> GSHMSSLPVPYKLPVSLSVGSCVIIKGTPIHSFINDPQLQVDFYTDMDEDSDI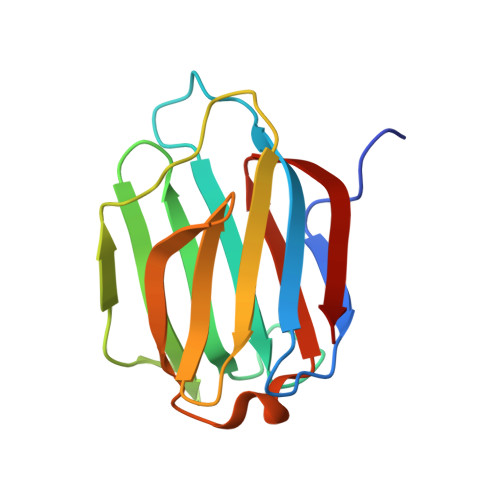AFRFRVHFGNHVVMNRREFGIWMLEETTDYVPFEDGKQFELCIYVHYNEYEIKVNGIRIYGFVHRIPPSFVKMVQVSRDISLTSVCVSN>MDEILARAGIFQGVEPSAIAALTKQLQPVDFPRGHTVFAEGEPGDRLYIIISGKVKIGRRAPDGRENLLTIMGPSDMFGELSIFDPGPRTSSATTITEVRAVSMDRDALRSWIADRPEISEQLLRVLARRLRRTNNNLADLIFTDVPGRVAKQLLQLAQRFGTQEGGALRVTHDLTQEEIAQLVGASR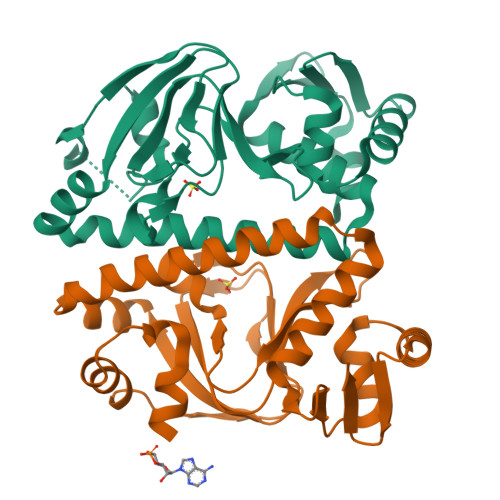ETVNKALADFAHRGWIRLEGKSVLISDSERLARRAR[2x]> GACLSIPNFPVHITGKTQQLHVGPKPSIARFSFNPFDLGTVFNRFQSLCAHLEGYSGDLIVNWLVTCSALTNARLYIIPVYDNYSFEKFSEEKLIQCKYEFKQISLVRKGTVHIPFVNWFGSYSRTRFPKLLFYFPNGVSGPSGEKIHVTVQLDRILNFSGLGHRLFKEIGPLVGE;> GSDPFSFLLNYSHCGTLVESSLNKGGMWCVPVSPVNLAAYTLQGEALVFNDAFVSKTHNWLHFMASTTAYWRGTLHYQMRVTYKDRNAACRNLVAFYTTNNESLFGFNNKPVGDTGISSVMGDSFSVDITVPFLIPTCYLQTIRGKFDYLNSCNGCIYFHLPTKSATSVQLWVRPGQDFDFARFRLLKAGYT;> GPDFTKIIWPTVVERNFSNPQSEITTTLQELYGDTFETVSICPPQSYGGELLKGKIFFSSTPEFTREDLVEGKILASFKLDEVLSGLGMGAMLMTQIMSGHATIRVSAKVMLSKFCSFALKLVYDELMQLNSDTTDFGKISVLPGAIFSTQEEEFSFDFELFSPGVHLKFDNNKLLGKVHLAALSAPNLTENMPESFSCTFNFSIVDVKTTFYNIGQ

Apple-latent spherical virus (ALSV) is a picorna-like plant virus found in apple leaves. The virions of ALSV consist of three proteins, Vp25, Vp20, and Vp24, and they show only a weak sequence homology to other virus capsid proteins. One protomer is made of Vp25, Vp20, and Vp24 subunits, and 60 copies of this unit compose one virion. The structure reveals that the three capsid proteins have characteristic jellyroll folds that contribute to capsid stabilization.

We have determined the structure of ALSV at 2.87-Å resolution by single-particle cryo-EM with a cold-field emission beam, which allowed de novo modeling of atomic coordinates on the cryo-EM map from a relatively smaller number of particle images with an improved B factor for map sharpening. The cryo-EM map revealed side-chain densities, and allowed de novo modeling for the whole virus capsid, except for three short segments (41–55, 100–116, and 146–151) in Vp24 and several residues in the N- and C-termini. The Vp24 subunits form a pentameric protrusion around a fivefold axis, and the protrusion sits on a base of Vp25 and Vp20. One of the striking features is an ~120-Å-long N-terminal extension of Vp25. The long extension has intimate hydrogen bonds with Vp20 (0Vp20) and the main body of Vp25 (2Vp25), and forms β-sheets with them (between β1 of 0Vp25 and β9 of 2Vp25, and between β2 of 0Vp25 and β8 of 0Vp20). In contrast, a smaller number of hydrogen bonds are found with Vp24. Thus, Vp25 and Vp20 have rather extensive interactions with their neighbors, and Vp24, which forms the pentameric protrusion, is more loosely held. Also, there is a hump or protuberance of genome density beneath each pentameric protrusion of the capsid and a pore with a diameter of ~4 Å there. The structure of ALSV and observations reported here suggest how the virion is stabilized and points to a possible mechanism for genome release through opening of weakly interacting Vp24 subunits.>SNAAHLPKVAQSFLNLLCAQTSLTFSIVVLDEHEVVPVARSYLPQQDNRVSPYGMHLGNRLPAHATSTGKVLLSVLDREVQIEWIEKYGLKRLTPYTITDEHTFLETLDAVRQSDYCLSTEEHELGVIAIAVPVLNAQ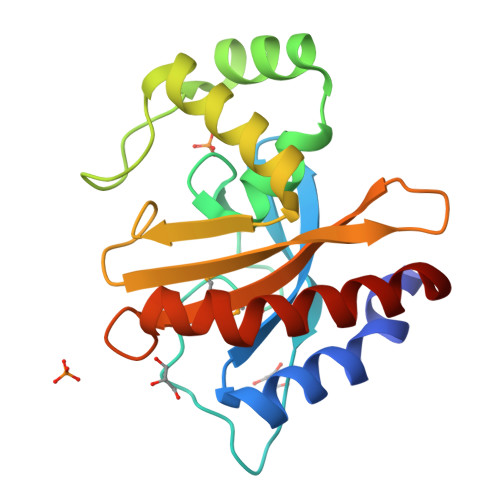GLTIAALNCMSQTNRVQPQYLIDQVLPLLRNTANELRNLV[3x]>MSEITLGKYLFERLKQVNVNTVFGLPGA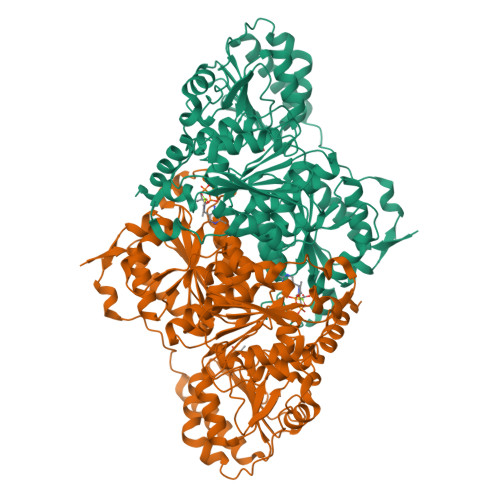FNLSLLDKIYEVEGMRWAGNANELNAAYAADGYARIKGMSCIITTFGVGELSALNGIAGSYAEHVGVLHVVGVPSISAQAKQLLLHHTLGNGDFTVFHRMSANISETTAMITDIATAPAEIDRCIRTTYVTQRPVYLGLPANLVDLNVPAKLLQTPIDMSLKPNDAESEKEVIDTILVLDKDAKNPVILADACCSRHDVKAETKKLIDLTQFPAFVTPMGKGSIDEQHPRYGGVYVGTLSKPEVKEAVESADLILSVGALLSDFNTGSFSYSYKTKNIVEFHSDHMKIRNATFPGVQMKFVLQKLLTAIADAAKGYKPVAVPARTPANAAVPASTPLKQEWMWNQLGNFLQEGDVVIAETGTSAFGINQTTFPNNTYGISQVLWGSIGFTTGATLGAAFAAEEIDPKKRVILFIGDGSLQLTVQEISTMIRWGLKPYLFVLNNDGYTIEKLIHGPKAQYNEIQGWDHLSLLPTFGAKDYETHRVATTGEWDKLTQDKSFNDNSKIRMIEVMLPVFDAPQNLVEQAKLTAATNAKQ[4x]>[2x]MASMTGGQQMG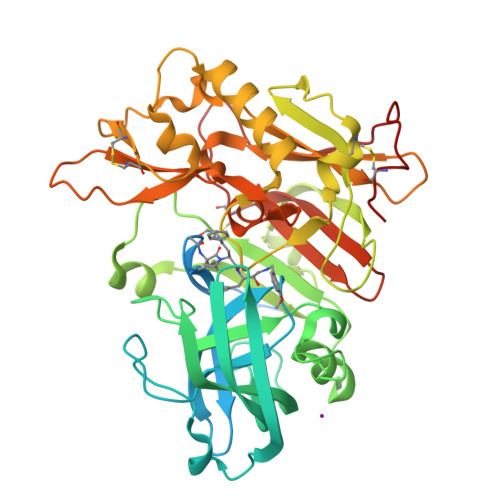RGSAGVLPAHGTQHGIRLPLRSGLGGAPLGLRLPRETDEEPEEPGRRGSFVEMVDNLRGKSGQGYYVEMTVGSPPQTLNILVDTGSSNFAVGAAPHPFLHRYYQRQLSSTYRDLRKGVYVPYTQGKWEGELGTDLVSIPHGPNVTVRANIAAITESDKFFINGSNWEGILGLAYAEIARPDDSLEPFFDSLVKQTHVPNLFSLQLCGAGFPLNQSEVLASVGGSMIIGGIDHSLYTGSLWYTPIRREWYYEVIIVRVEINGQDLKMDCKEYNYDKSIVDSGTTNLRLPKKVFEAAVKSIKAASSTEKFPDGFWLGEQLVCWQAGTTPWNIFPVISLYLMGEVTNQSFRITILPQQYLRPVEDVATSQDDCYKFAISQSSTGTVMGAVIMEGFYVVFDRARKRIGFAVSACHVHDEFRTAAVEGPFVTLDMEDCGYNIPQTDEST1-{(1R,2S)-2-HYDROXY-1-[2-(2-NAPHTHYLOXY)ETHYL]PROPYL}-1H-IMIDAZONE-4-CARBOXAMIDE | C19 H21 N3 O3 | 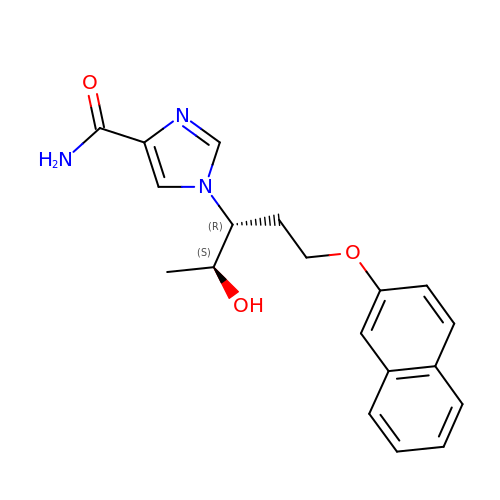UYAJDVNLQJVRHD-SCLBCKFNSA-N> SDLELHPPSYPWSHRGPLSSLDHTSIRRGFQVYKQVCSSCHSMDYVAYRHLVGVCYTEDEAKALAEEVEVQDGPNEDGEMFMRPGKLSDYFPKPY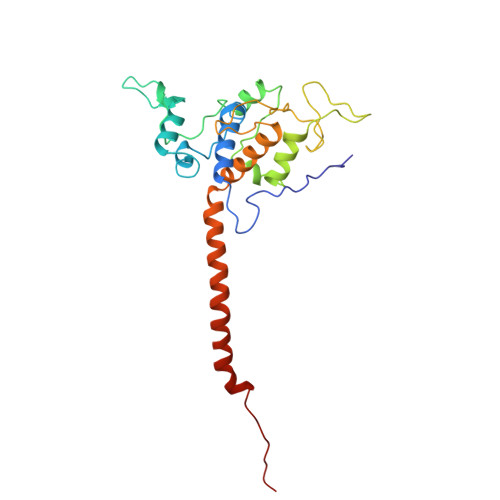PNPEAARAANNGALPPDLSYIVRARHGGEDYVFSLLTGYCEPPTGVSVREGLYFNPYFPGQAIGMAPPIYNDVLEFDDGTPATMSQVAKDVCTFLRWAAEPEHDHRKRMGLKMLLMMGLLVPLVYYMKRHKWSVLKSRKLAYRPPK>MSKLTTGSFSIEDLESVQITINNIVGAAKEAAEKAEEELGPMGPTPFPTAATVRDWSFTLFDRYEPVYTPMCDQCCYCTFGPCNLEGNRRGACGLDMKGQAAREFFLRCITGCACHSAHGRHLLDHIISIFGEDMPINMGASNVIAPNIQLITGRQPKTLGDLKPIMEYVEEELGQLLATVHAGQEGAAIDYDNKAMLAGILDHVGMEVSDIAQVTALGFPKSDPEAPLVEVGMGTLDASKPVIIAIGHNVAGVTYIMDYMEDNNLTDKMEIGGLCCTAFDMTRYKREDRKPPYAKIVGTISKELKVVRSGIPDVIVIDEQCVRADLVEEGKKLKIPVIASNEKVMYGLPDRTNDDVDAIIEDIKTGKIPGCVMLDYEKLGELVPRLAMEMAPLREGISAIPSDEEMASLVAKCVACGECALACPEELDIPDAIQAAKEGDFTALDFLHDLCVGCRRCEQVCNKEIPILSVIDKAAQKAIAEEKGLVRAGRGQVSDAEIRAEGLNLVMGTTPGVIAIIGCANYPAGSKDVYRIAEEFLNRNYIVAVSGCSAMDIGMYKDADGKTLYERFPGRFERGNILNTGSCVSNSHISGTCHKVAAIFAGRNLSGNLAEIADYTLNRVGAVGLAWGAYSQKAAAIGTGCNMYGIPAVLGPHSGKYRRALIAKTYDENKWKVYDSRNGSELDIPPSPEFLITTAETWQEACVLLAKNCIRPSDNNMGRSIKLTHWIELSEKYLGVLPEDWWKFVRHEADLPLSRREELLKKLETEHGWEIDWKKKKIISGPKIKFDVSSQPTNLKRLCKEA[2x];>[2x]MVDTTKNTKLFTSYGVKTSKAITTEVAAKLISKAKRPLFVVGTGVLDPELLDRAVKIAKAKNIPIAATGSSMPGFVDKDVNAKYINLHQLGFYLTDPDWPGLDGNGNYDTIILLGHKKYYINQVLSAVKNFSDVKSISIDRNYIQNATMSFGNLSKADHIAALDEVIDLL;>MSEFPFEISPMFEGERVRKEGMFVELGGPKSLGLELVRAKPMDEIEDGKVTIVGPDLKDMEEGKTYPWAMIFHVGGELVEPDLESVIERRVHDFINYCQGIMHLNQRYDVWMRISKDTAAKMDSFEPFGKAVMMLFKTELPFIEKMQVTFYTDQAEVEKQMAEAMEIFKARDARTKDLHDEDVDVFYGCTLCQSFAPTNVCVVSPDRVSLCGAINWFDGRAAAKVDPEGPQFAIEKGELLDAKTGEYSGVNEVAKKLSSGEFDKIKLHSFFDAPHTSCGCFEVVGFYIPEVDGIGWVNREYQGMAPNGLGFSTMAGQTGGGKQIVGFLGIGINYFYSPKFIQADGGWNRVVWLPSMLKEKIDEAIPDDMKDKIATEKDVTDIESLKTFLKEKNHPVVANWAAEAEEEEEEEEEEEEVAAEAAPMMMPAAGFQMPAMPAMPMMSGGAGGIKLTFKNAKITIDRMIISEKKEKK[2x]

Carbon monoxide dehydrogenase (CODH) and acetyl-CoA synthase (ACS) play major roles in the global carbon cycle through the consumption of CO and CO2 gases, production of acetate, and breakdown of acetate for methane generation. By contrast, methanogenic archaea employ four copies of CODH (α2ε2 heterotetramers) and eight copies of ACS (β monomers) that interact stably with eight copies of CFeSP (γδ heterodimers) to form a massive 2.2 MDa complex called the acetyl-CoA decarbonylase/synthase (ACDS) complex. ACDS plays a central role in that process, wherein the A-cluster of ACS cleaves acetyl-CoA into CO and a methyl moiety, the C-cluster of CODH oxidizes CO to CO2, and the corrinoid of CFeSP receives the methyl moiety, which is reduced to methane in downstream methanogenic metabolism. Through plunge freezing of the ACDS complex, we captured multiple subcomplexes including a CODH tetramer, a CODH/ACS pentamer, and a CODH/ACS hexamer and characterized these subcomplexes via cryogenic electron microscopy (cryo-EM).

With the next-generation chameleon instrument, different dissociation behavior led to formation of (α2ε2)β and (α2ε2)β2 CODH/ACS subcomplexes in addition to the α2ε2 CODH subcomplexes, allowing us to capture methanogenic CODH/ACS subcomplexes. Additionally, from the chameleon-plunged specimen, structures of the MetCODH/ACS pentamer and hexamer were determined, each at a global resolution of 3.2 Å. The structures reported here reveal that both A2 and A3 of ACS contact CODH. On CODH, the interaction surface is formed largely by Rossmann fold 2. Interestingly, the C-terminal extension of MetCODH, which differs from the C terminus of non-methanogenic CODHs, interacts with ACS. In the structure of MetCODH/ACS, we observe density consistent with CO binding to the proximal nickel of the A-cluster. The environment surrounding the CO-bound A-cluster of MetCODH/ACS is remarkably similar to that of MoorCODH/ACS. Substituting for Ile146, Val149, and Phe229 of the A1 domain of MoorACS are Leu504, Val507, and Phe601 of Rossmann fold 2 in MetCODH, respectively. Upon performing cavity calculations on the MetCODH/ACS complex, we see that this enzyme uses channel 2, like CaCODH/ACS, but MetCODH/ACS uses the channel 2B branch. In our structure of MetCODH/ACS, the channel between the C-cluster and A-cluster is open and resembles the open channel near the A-cluster in MoorCODH/ACS.Adeno-associated viruses (AAVs) belong to the Dependoparvovirus genus within the Parvoviridae family. Because of the broad differences in their tissue tropism and transduction efficiency and the absence of pathology, AAVs are the promising vehicles for therapeutic gene delivery. Adeno-associated virus receptor (AAVR), which is a glycosylated protein containing five polycystic kidney disease (PKD) repeat domains in its extracellular portion, was recently identified as a key proteinaceous receptor for multiple AAV serotypes to employ the post-attachment events of viral entry. To dissect the divergent rules of engagements between multiple AAV serotypes with AAVR, we select two AAV serotypes, AAV1 and AAV5, and solve the atomic structures of their complexes with AAVR by cryo-EM.

Meanwhile, the AAV1 and AAV5 particles alone were treated under identical conditions to obtain the unbound structures to identify potential conformational shifts upon receptor binding. The cryo-EM micrographs indicate the presence of AAVR on the AAV1 and AAV5 capsids, but at distinct positions. The final resolutions of the cryo-EM reconstruction were estimated by the FSC 0.143 cutoff to be 3.07 Å for AAV1 alone, 3.30 Å for the AAV1-AAVR complex, 3.18 Å for AAV5 alone, and 3.18 Å for the AAV5-AAVR complex. However, the structures of AAV5 capsomers with and without PKD1 attached display strict structural homology with an r.m.s.d of 0.27 Å for all Cɑ atoms from 519 residues, indicating that no obvious structural shift occurs upon AAVR binding. In this region, the conformation of the βGH7-ɑGH8 loop in AAV5 is more extended than the βGH6-αGH6′ loop in AAV2 and the βGH4-αGH5 loop in AAV1. Particularly, this part on the AAV5 capsid has a remarkable larger loop region shadowing the SIA binding pocket. There are two SIA-binding sites found on the AAV5 capsid, but only site A play essential role for AAV5 transduction. Notably, the structures of site A on the AAV5 capsid and the corresponding regions on the AAV1 and AAV2 capsids display high similarities. AAV5 is distinct among the dependent parvoviruses, since it was originally isolated from a patient sample instead of from laboratory stocks of adenovirus and has unique sequence and biochemical features.

> DGVGNASGDWHCDSTWMGDRVVTKSTRTWVLPSYNNHQYREIKSGSVDGSNANAYFGYSTPWGYFDFNRFHSHWSPRDWQRLINNYWGFRPRSLRVKIFNIQVKEVTVQDSTTTIANNLTSTVQVFTDDDYQLPYVVGNGTEGCLPAFPPQVFTLPQYGYATLNRDNTENPTERSSFFCLEYFPSKMLRTGNNFEFTYNFEEVPFHSSFAPSQNLFKLANPLVDQYLYRFVSTNNTGGVQFNKNLAGRYANTYKNWFPGPMGRTQGWNLGSGVNRASVSAFATTNRMELEGASYQVPPQPNGMTNNLQGSNTYALENTMIFNSQPANPGTTATYLEGNMLITSESETQPVNRVAYNVGGQMATNNQSSTTAPATGTYNLQEIVPGSVWMERDVYLQGPIWAKIPETGAHFHPSPAMGGFGLKHPPPMMLIKNTPVPGNITSFSDVPVSSFITQYSTGQVTVEMEWELKKENSKRWNPEIQYTNNYNDPQFVDFAPDSTGEYRTTRPIGTRYLTRPL> MATTTSNMFLYSLTIQPPTTITQALLGQFSGTKEQQIITASGSRLTLLQPDPRQGKVNTIVSHDIFGIIRAMAAFRLAGSHKDYIILATDSGRIAIIEYLPKENRFQRIHLETFGKSGVRRVIPGQYLAADPKGRACLIASVEKNKLV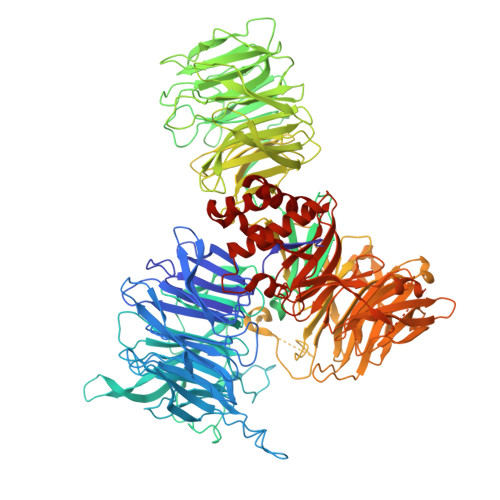YVLNRNAQAELTISSPLEAHKPGVIVLSLVALDVGYSNPVFAALEYEYSEADQDPTGQAAKQLEMQLVYYELDLGLNHVVRKWSDTVDPTSSLLFQVPGGNDGPSGVLVCGEENITYRHSNQEAFRVPIPRRRGATEDPNRKRTIVAGVMHKLKGSAGAFFFLLQTEDGDLFKVTIDMVEDEKGNPTGEVKRVKIKYFDTVPIAHSLCILKSGFLFVASEFGNHHFYQFEKLGDDDDEPEFTSDDFPADWNAPYNPVYFKPRPLENLVLVESIDSMNPLVGCKVANLTGEDAPQIYAICGNGARSSFRMLKHGLEVSEIVASELPGTPSAVWTTKLTKYDEYDAYIVLSFTNATLVLSIGETVEEVSDSGFLTTVPTLAVQQMGEEGLIQIHPKGIRHIVQGRVNEWPAPQHRSIVAATTNENQVVIALSSGEIVYFEMDADGSLAEYDEKKQMSGTVTSLSLGKVPEGLRRSSFLAVGCDDCTVRILSLDPESTLEMKSIQALTAAPSSLLIMSMEDSTGGTTLYLHIGLHSGVYLRTVLDEITGELTDTRQKFLGPKPTKLFQVTVQNQTCVLALSSRPWLGYTAPITRNFVMTPLSYTELGYTWSFNSEQCQEGMVGIHANYLRIFTIEKLGQTMIQKSCPLTYTPKRLVKHPEQPYFYVIEADNNTLPPELRAQLLEQSGAVNGDATVLPPEDFGYPKARGRWASCIEIVDPVSEEQPRVLKRIELEGNEAAVSAAVVPFASQDGESFLIVGTGKDMVLNPRASTEGAIHVYRFIDDGRDLEFIHKTIIEEPPLAFCPFQGRLLAGIGKMLRIYDLGLKQLLRKAQAEVSPQLIVSLDTRHNRIVVGDVQHGMTYVVYKPDSNKLIPFADDTIARWTTCTTMVDYESVAGGDKFGNLWIVRCPERASLESDEPGSEVQLLHARPYLHGAPNRLDLMAHFYPQDLPTSICKTNLVVGGQDVLVWSGIQGTVGVLIPFVTREDADFFQNLESHMRAEDPPLAGRDHLIYRGYYVPVKGVIDGDLCERFTLLPNDKKQMIAGELDRSVREIERKISDIRTRSAF3-[(~{E})-[2-methyl-3-oxidanyl-5-(phosphonooxymethyl)pyridin-4-yl]methylideneamino]oxypropanoic acid | C11 H15 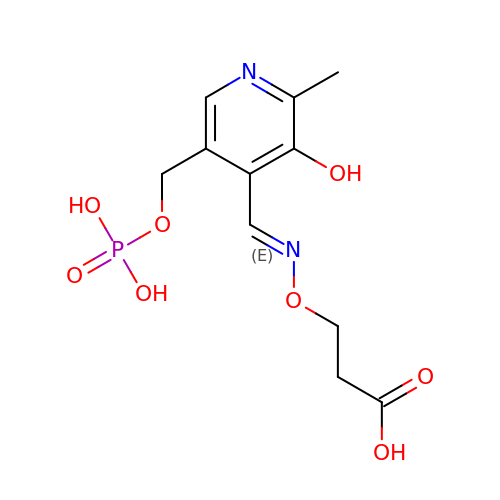N2 O8 P | WFKOVQOIGDESOJ-WLRTZDKTSA-N> SGSPSYTENKPDKKKKYMINDAKTIQLVGPLISSPDNLGFQKRSHKARELPRFLINQEPQLEKRAFVQDPWDKANQEKMISLEESIDDLNELYETLKKMRNTERSIMEEKGLVDKADSAKDLYDAIVFQGTCLDMCPTFERSRRNVEYTVYSYEKNQPNDKKASRTKALKVFARPAAAAAPPLPSDVRPPHILVKTLDYIVDNLLTTLPESEGFLWDRMRSIRQDFTYQNYSGPEAVDCNERIVRIHLLILHIMVKSNVEFSLQQELEQLHKSLITLSEIYDDVRSSGGTCPNEAEFRAYALLSKIRDPQYDENIQRLPKHIFQDKLVQMALCFRRVISNSAYTERGFVKTENCLNFYARFFQLMQSPSLPLLMGFFLQMHLTDIRFYALRALSHTLNKKHKPIPFIYLENMLLFNNRQEIIEFCNYYSIEIINGDAADLKTLQHYSHKLSETQPLKKTYLTCLERRLQKTTYKGLINGGED;> MDMANQLLDELAHGNFSHLTLNLSQNGREIAILQKQLTGFDDKQLETFVEQHPAMPNDTRFKIMCTSFLNYARDVDPWSAWSSSDLIFEFYQCLINCLINDNAPHIEMLIPVATRETEFIINLAGKLDSFHLQLHTRSHQFLSHISSILSRLFNSIKPPRGNASSTNIPGKQRILLYLVNKLNNIYFRIESPQLCSNIFKNFQPKSMLAHFNEYQLDQQIEYRYLLGRYYLLNSQVHNAFVQFNEAFQSLLNLPLTNQAITRNGTRILNYMIPTGLILGKMVKWGPLRPFLSQETIDNWSVLYKHVRYGNIQGVSLWLRQNERHLCARQLLIVLLEKLPMVTYRNLIKTVIKSWTTEWGQNKLPYSLIERVLQLSIGPTFEDPGAQEITIYNGIHSPKNVENVLVTLINLGLLRANCFPQLQLCVVKKTTMIQEIVPPVNERITKMFPAHSHVLW;> MSTDVAAAQAQSKIDLTKKKNEEINKKSLEEDDEFEDFPIDTWANGETIKSNAVTQTNIWEENWDDVEVDDDFTNELKAELDRYKRENQ

Transcription-export complex 2 (TREX-2, or THSC) facilitates localization of actively transcribing genes such as GAL1 to the nuclear periphery, contributes to the generation of export-competent mRNPs and influences gene expression through interactions with Mediator. TREX-2 is based on a Sac3 scaffold to which Thp1, Sem1, Cdc31 and Sus1 bind and consists of three modules: the N-region (Sac3∼1-100), which binds mRNA export factor Mex67:Mtr2; the M-region, in which Thp1 and Sem1 bind to Sac3∼100-550; and the CID region in which Cdc31 and two Sus1 chains bind to Sac3∼720-805. The juxtaposition of the winged helix motifs of Sac3 and Thp1, together with a surface patch of positive charge, contributes to the formation of a RNA-binding region in the TREX-2 complex.

Here we describe the 2.3 Å resolution crystal structure of a complex formed by Sac3 residues 60–550 complexed with Thp1 and Sem1. Crystals were obtained of the Sac360-550:Thp1:Sem1 complex that had P212121 symmetry with a = 78.2 Å, b = 84.1 Å, c = 165.5 Å and which diffracted to 2.3 Å resolution using synchrotron radiation. In addition to the previously determined structures of Thp1, Sem1 and Sac3 residues 255–551, Sac3 residues 82–255 were clear and easily traced, but reliable density corresponding to residues 60–81 was not observed, possibly indicating that this region was disordered. The Sac360-550:Thp1:Sem1 crystal structure indicated that the TPR-like repeats of Sac3 indeed extend to residue 137 and identified unequivocally the residues in the three major helices. However, the crystal structure showed that the residues that contributed to the three additional helices were 137–153, 157–177 and 205–213. These three additional helices both extend the TPR-like solenoid of the Sac3 M-region and also cap it. Remarkably, in the Sac360-556:Thp1:Sem1 complex crystals, Sac3 Arg256 was completely buried between the PCI region determined previously (residues 250–556) and the additional three helices (residues 137–250), where it formed a complex network of H-bonds to Asp293, Ser289 and Met203, and to Arg286, Ser289 and Lys238 through water S213 that was augmented with hydrophobic interactions with Ile256, Leu261 and Cys200. In addition to the three additional helices of the TPR-like repeat region, the crystal structure of the Sac360-556:Thp1:Sem1 complex showed that Sac3 residues 90–125 formed a remarkable extended loop that linked the distal region of the Sac3 TPR-like region to the N-terminal region of Thp1. The loop made extensive contacts with Thp1 and buried 1528 Å2 of surface area. However, the second positively charged cluster centered on Sac3 Arg256 that has been proposed to be involved in the interaction with Mediator was buried by the residues in the additional TPR region below residue 250 and so was inaccessible in the complete M-region structure.>[2x]MSPAKDVKVYKKILEQNKDIQDLLDKIVFDAQHGQIWFDENRMLLMHTSILGFL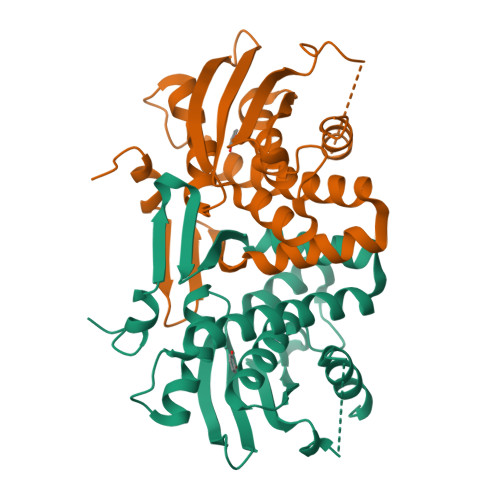RKDLYQMLGLERTKRFFIRCGYQAGMRDAEVTSKLRPNLNEAEAFMAGPQMHGIRGMVQVEVNELHLSHDLKQFYADFNWLNSFEAEVHLSEFGASDQPACWMLLGYACGYSSFVMGQTIIYQETHCVAQGDEHCRIIGKPLSEWENADELIRFMSPDAVSDEIIALQAELNQLK>HHHHHHHHGEVVSQRYPPAPGLLKYLEQDVCYSLYYYLNWTSLADCKTNFEETGISDVPSTVKVRCQSKNSIRFETEPSEHWQLFILMEHDNFDPIPFTLIEPNNVFGELITTANKEYQIWSTYLDEYGTLQDWMEGPIVLKFDQRNQQPDDIKYNVTQEFKYIILGNDSYTINGKFVWNTTGDRDLCFDIANICQNTNMKHAKI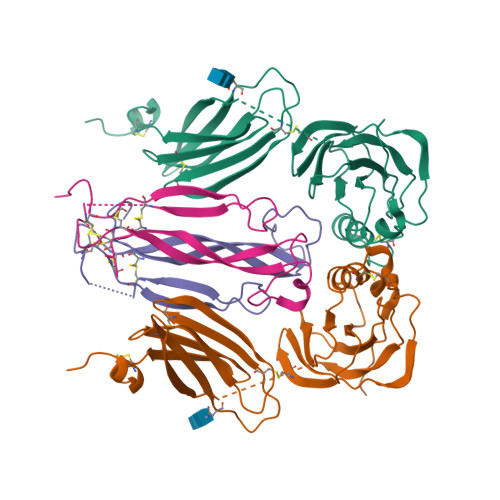WPTAHPSFDVENLVLNDECEIHVKGIHGTTKHKYKTPSCFELPECFLNNMEPEIPQDVAIAADQDLR[2x];>SLDQVENQAIPDPPCTCKYKKEIEDLGENSVPRFIETRNCQKTQQPTCRPPYICKESLYSITILKRRETKSQESLEIPNELKYRWVAESHPVSVACLCTRDYQLRYNNN[2x]(3R)-5-hydroxy-3-methyl-3-(phosphonooxy)pentanoic 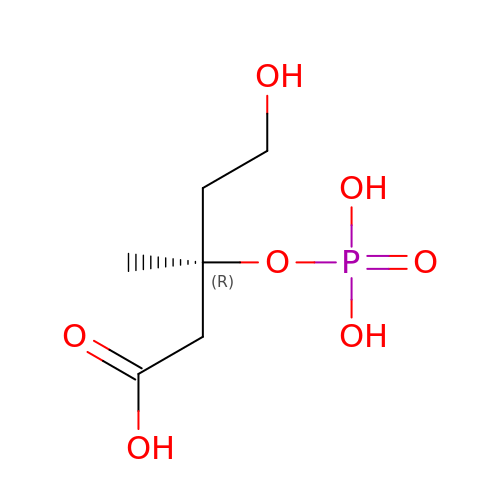acid | C6 H13 O7 P | VWCNCYQNEAUWMQ-ZCFIWIBFSA-N N-[(1R,2R,4R)-1-(cyclohexylmethyl)-2-hydroxy-6-methyl-4-{[(2R)-2-methylbutyl]carbamoyl}heptyl]-3-(1H-imidazol-3-ium-4-yl)-N~2~-[3-naphthalen-1-yl-2-(naphthalen-1-ylmethyl)propanoyl]-L-alaninamide 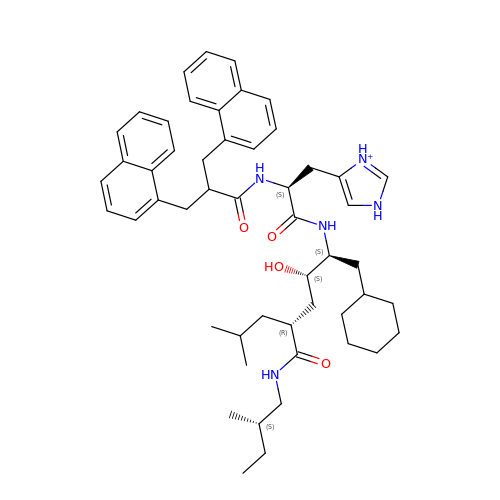| C51 H68 N5 O4 | SIGGSNKWBGJQQB-XNTVDALVSA-O>AAPKDHLIHNHHKHEHAHAEHLGGSAWSHPQFEKGSGLEVLFQGPAEFASSQGNDKAPKNLHLVKRNAIKTRPSDALGGLEPGDPAPAFQVHTLDGMFVYSPRNESGRALIVHAFTNKSAFLECLWTWSESLSDLLDYLPSSTEVLMLSMDETAEQDALWMREQVYRAAAHRGKEILSRLHFSPTHVYNLGNWIPRVLYSWGCGGHNCGLGQVVFSSPDWKGPVIGKRLNARYDWLYAHWSTDPYRLLDVGDGCAPVASLKGAVAWVSEGGCSFFTKIKNMEKSNATGVLVYALPGNNIQDMNCKGDECFTSLHIPASMVHFQPKVKEALQKGRPVNVKFQVTPSRSFFFGIDQRGVLSEMGWFLYPSFRFMAWQAQWFVFNDALLEQLSQPAVTVSVFDHHDMHGNAGAHAVVDLPADISPYDVLELDTSLSCPGRRDETCAHWDHTVQLFVCCNDSSPYCNQELGRWVTAFRRGTGHWLTDVSPLIPLLNNKKCSFTMKTAPWAMPWMTTLNLRFSQSNKTERLYPFEVMPLFNGGTFDKDYNRRYHEITFSIPAATKKVELYAVITGHGSDDNNCGEFCVTSHYFLINRSINNTLVFEAAGSPLGCSLLVPKGGVPNECGTWLYGRGGWCDGLQVDPWRRDITSQLDMSGSNSVRYFGLFEGRDPNPKTDPGNILMYSYLVFYQ[2x]

Peptide:N-glycanase (PNGase) is a deglycosylating enzyme acting on asparagine(N)-linked glycans on glycoproteins. The other is called acid PNGase and is found in fish embryos; it is active at acidic pH and is believed to be of lysosomal origin. In this study, we identified the gene encoding the acid PNGase, which we named Ngly2, in zebrafish (Danio rerio). Zebrafish Ngly2 exhibited maximal PNGase activity under acidic conditions, with the highest activity observed at pH 3.5.

The structure of zebrafish Ngly2 was determined by cryo-EM, showing that it forms homodimers and that its substrate is accommodated in the cleft between the protease-associated domain and PNGase domain, where the catalytic residues are located. The 3D reconstruction, conducted with imposed C2 symmetry, yielded a density map at an average nominal resolution of 2.7 Å. Structural homology analysis using the Dali server revealed that Ngly2 possesses two additional domains in the N-terminal region, located upstream of the PNGase domain. One of these domains, composed of residues 58 to 185 and 319 to 343, exhibits significant structural similarity to a thioredoxin-like (Tx-like) domain found in peroxiredoxins. The other region, spanning residues 186 to 318, is identified as a protease-associated (PA) domain, showing structural similarity to domains found in certain peptidases. Ngly2 homodimerizes primarily through interactions between the Tx-like and PA domains. Around the twofold axis, the Tx-like domains dimerize via extensive hydrophobic interactions, burying approximately 1500 Å2 of solvent-accessible surface area upon dimer formation. The domain consists of two jelly-roll subdomains stabilized by hydrophobic core residues and disulfide bonds. Its overall structure is nearly identical to that of PNGase F, and the catalytic residues essential for the enzymatic activity are conserved in Ngly2 (Asp421 and Glu555) (asterisks in Figs. S2; 3C). In contrast, Trp59 and Arg61 are replaced by histidines, His422 and His546, respectively. These histidines could form hydrogen bonds with the chitobiose via protonated imidazole groups.>GSHMKLNKYIDHTILKPETTQEQVEKILAEAKEYDFASVCVNPTWVALAAESLKDSDVKVCTVIGFPLGANT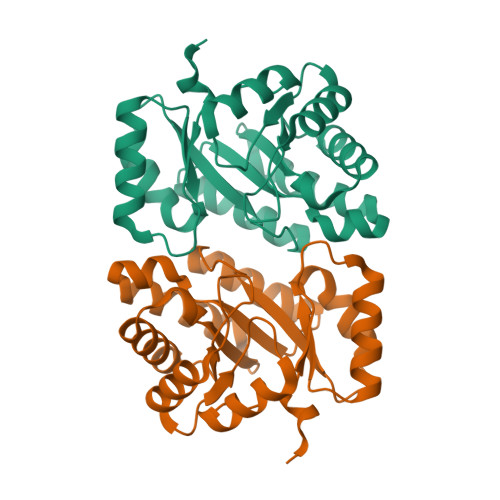PAVKAFETKDAISNGADEIDMVINIGALKTGNYDLVLEDIKAVVAASGDKLVKVIIEACLLTDDEKVKACQLSQEAGADYVKTSTGFSTGGATVADVALMRKTVGPDMGVKASGGARSYEDAIAFIEAGASR[12x]>SAVKAARYGKDNVRVYKVHKDEKTGVQTVYEMTVCVLLEGEIETSYTKADNSVIVATDSIKNTIYITAKQNPVTPPELFGSILGTHFIEKYNHIHAAHVNIVCHRWTRMDIDGKPHPHSFIRDSEEKRNVQVDVVEGKGIDIKSSLSGLTVLKSTNSQFWGFLRDEYTTLKETWDRILSTDVDATWQWKNFSGLQEVRSHVPKFDATWATAREVTLKTFAEDNSASVQATMYKMAEQILARQQLIETVEYSLPNKHYFEIDLSWH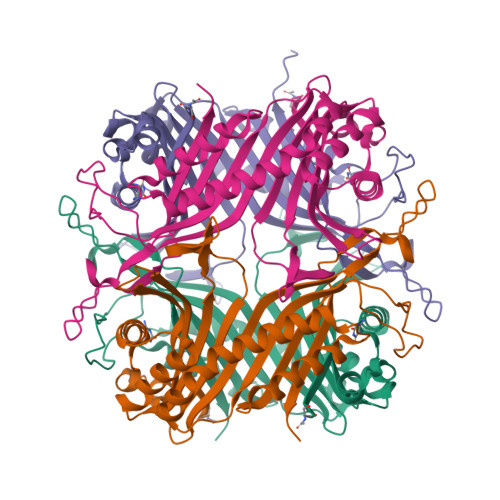KGLQNTGKNAEVFAPQSDPNGLIKCTVGRSSLKSKL[4x]> MSTNKSEPTRKVDVHLTDNGTPFAYSMTSHKNVKVRAEVQPPLQLPGLIIFVHGVNSEGEWYDYAERSLCAGLNQRLGLEGEHGLKENNYEGGFFVNSDKSEGGWEHTYEIEGSQKKWVSGPRKITKGGDGRSPVIRFYWGYRAADNETDTYAIPLKNKKGDNYYDLPPESRKAKGPWFWGGGPFQNGCNQLVSLWSKTGFNNNPSLLGVPLPFSTQVLNGERDRLLSDAPPRHYYAHAAGRLAKLIKTIRNQHPEDTVTVLSHSQGTMIALAAAAIEAPDALFVMNSPYALENEPTTYISYPIKEIISRKARSATFADIVKKVAENKTRLKQQGCDNLLAGMSSDGNSWIPEGKTHNGLPERDNHGTTWIYCNPHDRVMGSS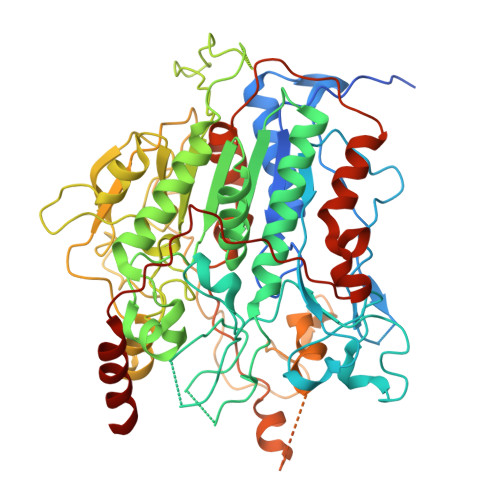PLRSIGWQGLPDTKDGTPHTLFKQAGDTLYVRILGRNTPCGGTPTAQTHFSNLGDGKPFWDSTTTLLQRATWPDPDSGQTLTINAPQVPEPLTAEELKNFDQDYARDEKQSGGAGYAYGQINPETKKPVDTDYRYYISLYGYFDRKMVPKKDSGYYQSGPGSKEDRVKYEKQSQEEMLEEVRTYVQRPTDHSTLPSDERFMSRVVAYDLPIGYCWHSWDKAGLEELRRQADWLESDDYYFSGKLTVPPIPPAIKQDVAEDAEQRKAEEKARLRNV> MHHHHHHTAVQLIVGLGNPGPEYDQTRHNAGALFVERLAHAQGVSLVADRKYFGLVGKFSHQGKDVRLLIPTTYMNRSGQSVAALAGFFRIAPDAILVAHDELDMPPGVAKLKTGGGHGGHNGLRDIIAQLGNQNS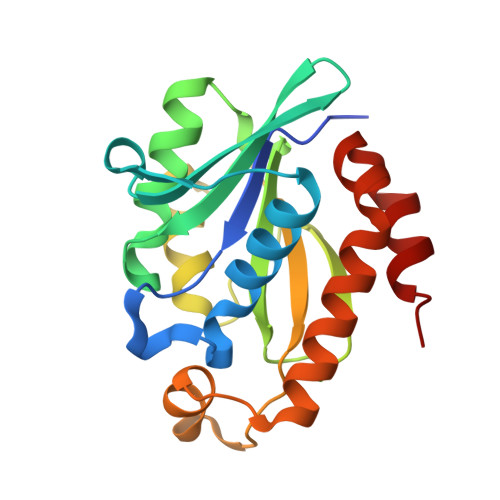FHRLRLGIGHPGHSSLVSGYVLGRAPRSEQELLDTSIDFALGVLPEMLAGDWTRAMQKLHSQK> MNEYAPLRLHVPEPTGRPGCQTDFSYLRLNDAGQARKPPVDVDAADTADLSYSLVRVLDEQGDAQGPWAEDIDPQILRQGMRAML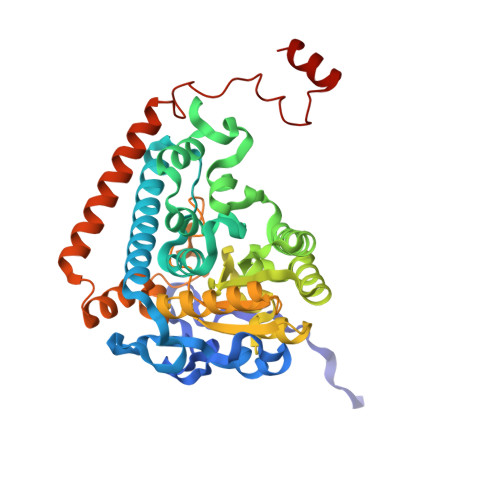KTRIFDSRMVVAQRQKKMSFYMQSLGEEAIGSGQALALNRTDMCFPTYRQQSILMARDVSLVEMICQLLSNERDPLKGRQLPIMYSVREAGFFTISGNLATQFVQAVGWAMASAIKGDTKIASAWIGDGATAESDFHTALTFAHVYRAPVILNVVNNQWAISTFQAIAGGESTTFAGRGVGCGIASLRVDGNDFVAVYAASRWAAERARRGLGPSLIEWVTYRAGPHSTSDDPSKYRPADDWSHFPLGDPIARLKQHLIKIGHWSEEEHQATTAEFEAAVIAAQKEAEQYGTLANGHIPSAASMFEDVYKEMPDHLRRQRQELGV> SNAVGFAPELYCGLENCYDVLEVNREEFDKQKLAKAYRALAR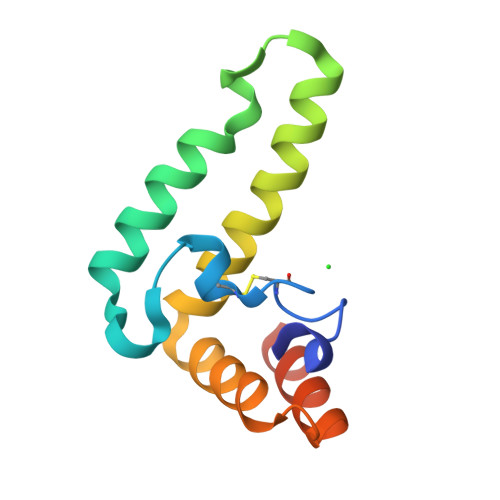KHHPDRVKNKEEKLLAEERFRVIATAYETLKDDEAKTNYDYYLDHPDQRFYNYYQYYRLRAAPKVDL>MGAMAYPLLLCLLLAQLGLGAVGASRDPQGRPDSPRERTPKGKPHAQQPGRASASDSSAPWSRSTDGTILAQKLAEEVPMDVASYLYTGDSHQLKRANCSGRYELAGLPGKWPALASAHPSLHRALDTLTHATNFLNVMLQSNKSREQNLQDD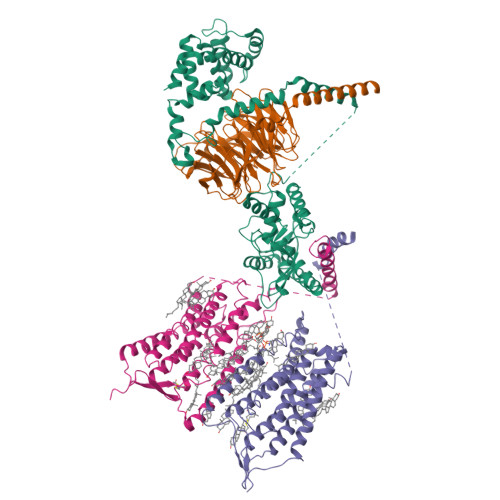LDWYQALVWSLLEGEPSISRAAITFSTDSLSAPAPQVFLQATREESRILLQDLSSSAPHLANATLETEWFHGLRRKWRPHLHRRGPNQGPRGLGHSWRRKDGLGGDKSHFKWSPPYLECENGSYKPGWLVTLSSAIYGLQPNLVPEFRGVMKVDINLQKVDIDQCSSDGWFSGTHKCHLNNSECMPIKGLGFVLGAYECICKAGFYHPGVLPVNNFRRRGPDQHISGSTKDVSEEAYVCLPCREGCPFCADDSPCFVQEDKYLRLAIISFQALCMLLDFVSMLVVYHFRKAKSIRASGLILLETILFGSLLLYFPVVILYFEPSTFRCILLRWARLLGFATVYGTVTLKLHRVLKVFLSRTAQRIPYMTGGRVMRMLAVILLVVFWFLIGWTSSVCQNLEKQISLIGQGKTSDHLIFNMCLIDRWDYMTAVAEFLFLLWGVYLCYAVRTVPSAFHEPRYMAVAVHNELIISAIFHTIRFVLASRLQSDWMLMLYFAHTHLTVTVTIGLLLIPKFSHSSNNPRDDIATEAYEDELDMGRSGSYLNSSINSAWSEHSLDPEDIRDELKKLYAQLEIYKRKKMITNNPHLQKKRCSKKGLGRSIMRRITEIPETVSRQCSKEDKELEVLFQ[2x];> MAQGNNYGQTSNGVADESPNMLVYRKMEDVIARMQDEKNGIPIRTVKSFLSKIPSVFSGSDIVQWLIKNLTIEDPVEALHLGTLMAAHGYFFPISDHVLTLKDDGTFYRFQTPYFWPSNCWEPENTDYAVYLCKRTMQNKARLELADYEAESLARLQRAFARKWEFIFMQAEAQAKVDKKRDKIERKILDSQERAFWDVHRPVPGCVNTTEVDIKKSSRMRNPHKTRKSVYGLQNDIRSHSPTHTPTPETKPPTEDELQQQIKYWQIQLDRHRLKMSKVADSLLSYTEQYLEYDPFLLPPDPSNPWLSDDTTFWELEASKEPSQQRVKRWGFGMDEALKDPVGREQFLKFLESEFSSENLRFWLAVEDLKKRPIKEVPSRVQEIWQEFLAPGAPSAINLDSKSYDKTTQNVKEPGRYTFEDAQEHIYKLMKSDSYPRFIRSSAYQELLQAKKKGKSLTSKRLTSLAQSY;> MATDGLHENETLASLKSEAESLKGKLEEERAKLHDVELHQVAERVEALGQFVMKTRRTLKGHGNKVLCMDWCKDKRRIVSSSQDGKVIVWDSFTTNKEHAVTMPCTWVMACAYAPSGCAIACGGLDNKCSVYPLTFDKNENMAAKKKSVAMHTNYLSACSFTNSDMQILTASGDGTCALWDVESGQLLQSFHGHGADVLCLDLAPSETGNTFVSGGCDKKAMVWDMRSGQCVQAFETHESDVNSVRYYPSGDAFASGSDDATCRLYDLRADREVAIYSKESIIFGASSVDFSLSGRLLFAGYNDYTINVWDVLKGSRVSILFGHENRVSTLRVSPDGTAFCSGSWDHTLRVWA>[4x]MSQHNEKNPHQHQSPLHDSSEAKPGMDSLAPEDGSHRPAAEPTPPGAQPTAPGSLKAPDTRNEKLNSLEDVRKGSENYALTTNQGVRIADDQNSLRAGSRGPTLLEDFILREKITHFDHERIPERIVNARGSAAHGYFQPYKSLSDITKADFLSDPNKITPVFVRFSTVQGGAGSADTVRDIRGFATKFYTEEGIFDLVGNNTPIFFIQDAHKFPDFVHAVKPEPHWAIPQGQSAHDTFWDYVSLQPETLHNVMWAMSDRGIPRSYRTMEGFGIHTFRLINAEGKATFVRFHWKPLAGKASLVWDEAQKLTGRDPDFHRRELWEAIEAGDFPEYELGFQLIPEEDEFKFDFDLLD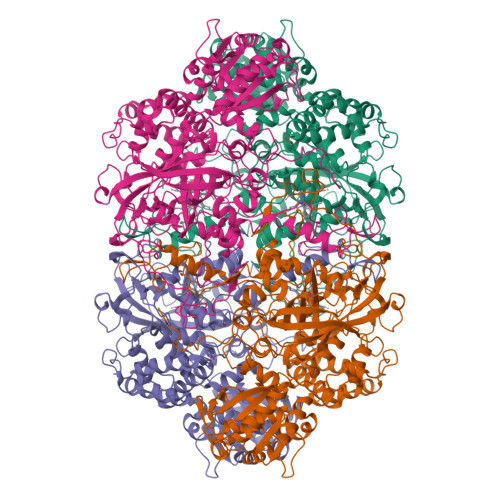PTKLIPEELVPVQRVGKMVLNRNPDNFFAENEQAAFHPGHIVPGLDFTNDPLLQGRLFSYTDTQISRLGGPNFHEIPINRPTCPYHNFQRDGMHRMGIDTNPANYEPNSINDNWPRETPPGPKRGGFESYQERVEGNKVRERSPSFGEYYSHPRLFWLSQTPFEQRHIVDGFSFELSKVVRPYIRERVVDQLAHIDLTLAQAVAKNLGIELTDDQLNITPPPDVNGLKKDPSLSLYAIPDGDVKGRVVAILLNDEVRSADLLAILKALKAKGVHAKLLYSRMGEVTADDGTVLPIAATFAGAPSLTVDAVIVPCGNIADIADNGDANYYLMEAYKHLKPIALAGDARKFKATIKIADQGEEGIVEADSADGSFMDELLTLMAAHRVWSRIPKIDKIPA> MELENYEQPVVLREDNRRRRRRMKPRSTAASLSSMELIPIEFVLPTSQRNTKTPETALLHVAGHGNVEQMKAQVWLRALETSVSADFYHRLGPDHFLLLYQKKGQWYEIYDKYQVVQTLDCLRYWKVLHRSPGQIHVVQRHAPSEETLAFQRQLNALIGYDVTDVSNVHDDELEFTRRRLVTPRMAEVAGRDPKLYAMHPWVTSKPLPEYLLKKITNNCVFIVIHRSTTSQTIKVSADDTPGTILQSFFTKMAKKKSLMDIPESQNERDFVLRVCGRDEYLVGETPIKNFQWVRQCLKNGEEIHLVLDTPPDPALDEVRKEEWPLVDDCTGVTGYHEQLTIHGKD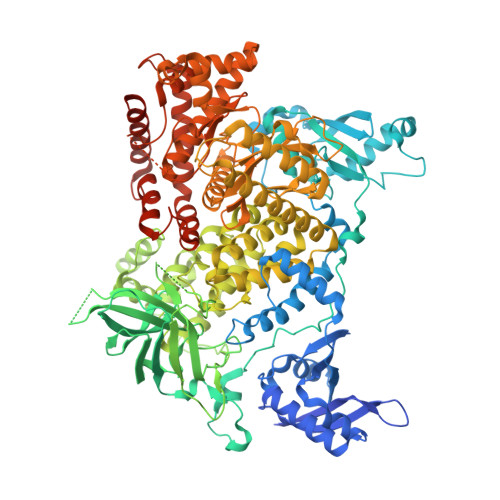HESVFTVSLWDCDRKFRVKIRGIDIPVLPRTADLTVFVEANIQYGQQVLCQRRTSPKPFTEEVLWNVWLEFSIKIKDLPKGALLNLQIYCGKAPALSGKTSAEMPSPESKGKAQLLYYVNLLLIDHRFLLRHGEYVLHMWQLSGKGEDQGSFNADKLTSRTNPDKENSMSISILLDNYCHPIALPKHRPTPDPEGDRVRAEMPNQLRKQLEAIIATDPLNPLTAEDKELLWHFRYESLKDPKAYPKLFSSVKWGQQEIVAKTYQLLAKREVWDQSALDVGLTMQLLDCNFSDENVRAIAVQKLESLEDDDVLHYLLQLVQAVKFEPYHDSALARFLLKRGLRNKRIGHFLFWFLRSEIAQSRHYQQRFAVILEAYLRGCGTAMLHDFTQQVQVIDMLQKVTIDIKSLSAEKYDVSSQVISQLKQKLENLQNLNLPQSFRVPYDPGLKAGALVIEKCKVMASKKKPLWLEFKCADPTALSNETIGIIFKHGDDLRQDMLILQILRIMESIWETESLDLCLLPYGCISTGDKIGMIEIVKDATTIAKIQQSTVGNTGAFKDEVLSHWLKEKCPIEEKFQAAVERFVYSCAGYCVATFVLGIGDRHNDNIMISETGNLFHIDFGHILGNYKSFLGINKERVPFVLTPDFLFVMGTSGKKTSLHFQKFQDVCVKAYLALRHHTNLLIILFSMMLMTGMPQLTSKEDIEYIRDALTVGKSEEDAKKYFLDQIEVCRDKGWTVQFNWFLHLVLGIKQGEKHSA>[2x]TETTSFLITKFSPDQQNLIFQGDGYTTKEKLTLTKA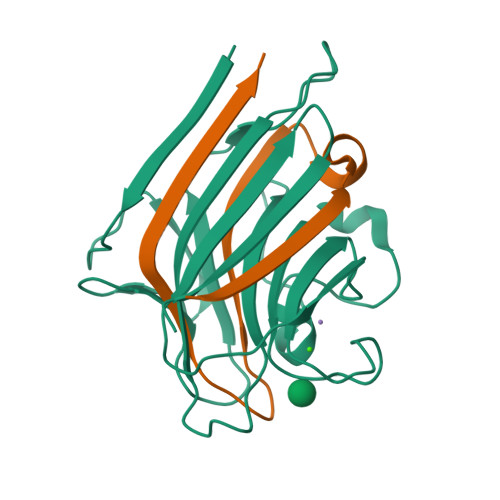VKNTVGRALYSSPIHIWDRETGNVANFVTSFTFVINAPNSYNVADGFTFFIAPVDTKPQTGGGYLGVFNSAEYDKTTQTVAVEFDTFYNAAWDPSNRDRHIGIDVNSIKSVNTKSWKLQNGEEANVVIAFNAATNVLTVSLTYPN;>VTSYTLSDVVSLKDVVPEWVRIGFSATTGAEYAAHEVLSWSFHSELS[2x]>[4x]AYSNTYQEFTNIDQAKAWGNAQYKKYGLSKSEKEAIVSYTKSASEINGKLRQNKGVINGFPSNLIKQVELLDKSFNKMKTPENIMLFRGDDPAYLGTEFQNTLL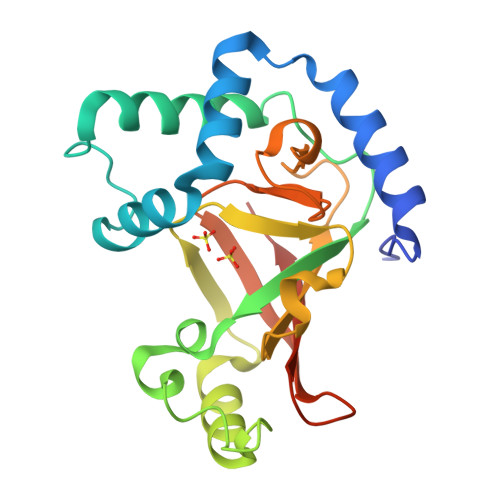NSNGTINKTAFEKAKAKFLNKDRLEYGYISTSLMNVSQFAGRPIITKFKVAKGSKAGYIDPISAFAGALEMLLPRHSTYHIDDMRLSSDGKQIIITATMMGTAINPK>[2x]SNANGDQQTMVYIV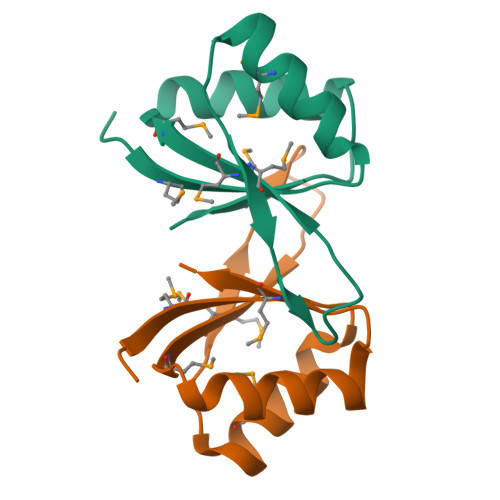SAKRKIIADRMLQELDLGVTMLQAVGAYKNNETEVIMCVMRKATLVKVRNLLKEVDPDAFMIVSTANEVFGEGFKNQYETEI>MYSDQTYEVIKNRTLENINLDIYKGEGSFLNNMVSGNNLELSKIYLELSKMHKMAFIQDTYNQFLDKRVNEFGVYRKLGTESNGEVEFIGEKGTVINNGTIISYRDLLFVVIKDVTIGSEEGDNSPVQALEVGKKYNLPTNCEFKLVDNISGVTKITNTRSFEGGTDIETDEELKERFYKIQRNQATSGNKAHYEEWALEVDGVYNVKVYPRWDGPGTVKVLIFGKNNQAVDTETIERCQQHIDEEKPIGPTITVVTPLPIEISISAVMKLEDGYTLDNVKESFLESINTYFRDIRGEIIYTKVMGILINTTGVHDLSNLLINGSTDNITINEDKIPSVTTVNFSEVENQ[12x];>MAIGLPSINISFKELATTVKERSARGIIAMVLKDAKALGLNEIHEKEDIPVDLSAENKEYINLALMGNVNTPNKLLVYVIEGEADIQTALDFLETKEFNYLCMPKAVEADKTAIKNWIIKLRDIDKVKVKAVLGKVVGNHEGIINFTTEDVLVGEKKYSVDEFTSRVAGLIAGTPLSQSVTYTKLSDVVDIPKMTKVDAESRVNKGELILIKEAGAIRIARGVNSLTELTAEKGEMFQKIKIVDTLDIIHSDIRKVIIDDYIGKVTNSYDNKCLLIVAIKSYLEELEKSALIESDSTVEIDFEAQKSYLKSKGVDLSYMTLQEIKEANTGSKVFLKAKIKVLDAMEDIDLSIEI[12x];>[6x]MSTIFPFIGVPEDYILPKTEELPIFREVAWDFEKDEPILEKGDFKIIEKKEALKVWIYKCIKTNRYEHEIYSLEYGTELSELIGQKYTKGLTESEASRFIKEALLINPYILEVNVKSANFNRDILSANVKVSTIYGEVEINV;>MKLIDKLPSFDRNYIVEEIQGAYDTELNILKEDIDDTFNQLFVDTATWGLDMWEDILCIEKKELDFDTRRSNIKAKMRSRGTSTIEVIKSICEAYTKSETDIKVYSDEFTFVLSFIANNCDYKTLLDCSDMIERVKPAHLLHYLEPIILDKSMVYCGGGMVCSEEVKVHPYFEPIIKCSAVVNCGAGMISREEIKVYPLSIKCIENNCKINIAIANDTGVENVVVYPKSEVV[6x];>[12x]MANMEARNVMSGTWGELWLDGNKVAEVKKFQAKMEFTKEDIIIAGQMGTDTKYMGYKGKGSITLYHVSSRMHKLIGEKIKRGSEPRFVAISKLNDPDSYGAERIAVKNIAFDDLTLADWEVGVKGEIEAPFTFTEYDFLDII;>MGNVREEGINMYLTDNYTPKMNQIISVTDNFRRATVAVSLSTNVMASSIKNSIGSASNRVNSLNSSLRKVQTTASSVSSTMTKLSSSINAVSGVIGSLNGSIMRLAITIAMIIDYFNKLIQKKNEFNSNIMIILIFKAKSDEVEKTKNKLLGNLKKIGGKIWNIVIKAKDMTKRVISSILGKLKQVEKRPYQGSINLKDMVSSAMGRILPKLMLFKNTFWSGVIAIKDMASGIISKVFPKLRLFAGKVWSGAIAVKDMASGILGSIKGKISDLTNGATIGVAVKKGVDLLGQEQNQKVVLESVMKRNTGKVNQIDVDDYYGSLVRMANDTPFDPEDVVAMGTKAKMISNITGGKKEKDITQAMVDVRALNMNTSSEQDVSAAFLSAAKGNMESLNTLVGENYKTFDEALEGISVKQMGLAKEMSNTIPGIISGAQTSINNGLKSIVKPFDDILGQGLKKIKTFIESGLGNLAGLSEKMAGKIGNVMNGKIIIGNKYDQMQSRSVKNGKEFSDSTQYRISNEAEKRKMMVENKQERFENHAATMIGNAPKAIVNAGSTLLQNIDFTALIDSLLPVVNLVNNLLDSINNKSPIAQGLISIFGTIVTTAFQLIGPVVEAVSPIITRIFTFLGEYAPQINNFIETLGVIWKTVWETLGPLLETGWKIIEPILGAFFNILDKVCKIVKDICKWWQTMINKIKNGSITGTVLNLVEKSKKNYKDNPYAGTKAGDSGKAYSGKKGNNAFGLNYVPYNDYQTRLHEGEMVLTKQEANQYRSRKNGGNINIAKLADTIVIREEADIEKITSKLVASIQLAQLGGVL[3x];>MANPINEFIGIIREEGKYHNQPSFFIGKIKSKLPDLKIETNNIILEKEDILIDSWMIDRQLETFDTETNQEHQHEVKNPFIDNFESGDMVIMFRIGEKFAVVSKLVSL[3x];>[6x]MEMWLRQAEDRFRFPVFPSSFSINGKAAVNSSSILKIGEIATFGGVALKSISISSFFPNKDYTFCDYTGFPSPYDCVNKIEKWMKEGFILRFTITETNINMEVIIEGFSYEERDGTRDVYFTLDLKEYKRIKIPKVTPKQ;>MIKIWVHIKNGSIYDITDIVDKVSWSGDYKSPSRTLEFSIIQSSFDNVFQQIDIPIASTVCFYVDEKELFRGMIINRSKDSSSNEISFVSKDMGFLLTQSEVSYNFKDKLVEDIAKQVFAENRLSVGIIAKTNVKYTKMFIGVNGYDTIMSAYTEASKKTKKKYMIEANLDKFNVIEKGTVTLSVMFEEGFNIINTTFSESMENVKNKVIVVDQYGSKISEKIDNEIFKEVNVIMQKVIQQQENQDVDIDSEFNGIEKSCSLKGYGDVSCITGRGVKVKDSYT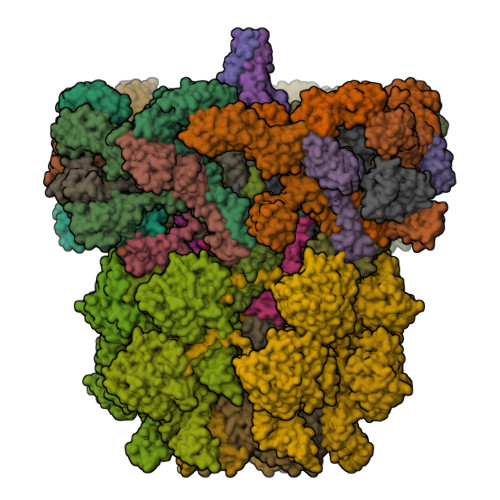KLVGLFYIDTDKHTWQNGEYQIELELNFQNLMDEKSAGQDEPKEESNLGGEDYAGGKEFTAEFTAYCPRKEEGGDTDCRKKKLDPSKKTCAAPMVGKYEQTYYTKEFLNKHPLLNYGDEIQVITGVSGRDGVYKVNDVGPAITIEKNGTYHIDILFGNVEEASKFGRRKGKIIIGGYSGNVSDKAKIVISEAKKHLGKPYKWGGNGPSSFDCSGLMVYCFKKVNVSLPRTSNQQSKKGKKVEQKNLQAGDLVFFHNPVSHVGLYIGNGEFLHAPQKGDVVKISKLSSRRDFNTARRVL[3x]> MPTVSVKRDLLFQALGRTYTDEEFDELCFEFGLELDEITSEKEIISKEQGNVKAAGASDVVLYKIDVPANRYDLLCLEGLVRGLQVFKERIKAPVYKRVMPDGKIQKLIITEETAKIRPFAVAAVLRNIKFTKDRYDSFIELQEKLHQNICRKRALVAIGTHDLDTLSGPFTYTAKRPSDIKFKPLNKTKEYT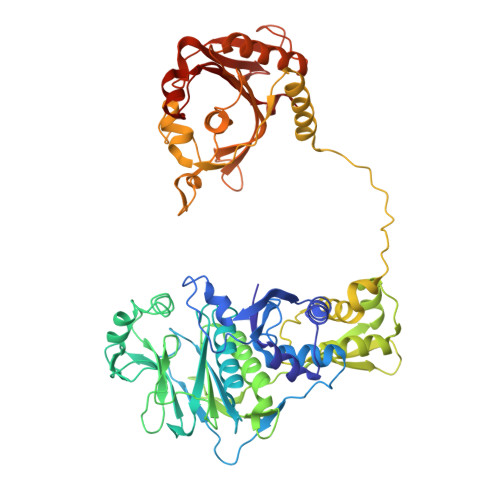ACELMNIYKTDNHLKHYLHIIENKPLYPVIYDSNGVVLSMPPIINGDHSRITVNTRNIFIECTGTDFTKAKIVLDIIVTMFSEYCENQFTVEAAEVVFPNGKSHTFPELAYRKEMVRADLINKKVGIRETPENLAKLLTRMYLKSEVIGDGNQIEIEIPPTRADIIHACDIVEDAAIAYGYNNIQMTLPKTYTIANQFPLNKLTELLRHDMAAAGFTEALTFALCSQEDIADKLGVDISATKAVHISNPKTAEFQVARTTLLPGLLKTIAANRKMPLPLKLFEISDIVIKDSNTDVGAKNYRHLCAVYYNKNPGFEIIHGLLDRIMQLLDVPPGEDKGGYVIKASEGPAFFPGRCAEIFARGQSVGKLGVLHPDVITKFELTMPCSSLEINIGPFL>SNAMKLASKTAIVTGAARGIGFGIAQVLAREGARVIIADRDAHGEAAAASLRESGAQALFISCNIAEKTQVEALFSQAEEAFGPVDILVNNAGINRDAMLHKLTEADWDTVIDVNLKGTFLCMQQAAIRMRERGAGRIINIASASWLGNVGQTNYSASKAGVVGMTKTACRELAKKGVTVNAICPGFIDTDMTRGV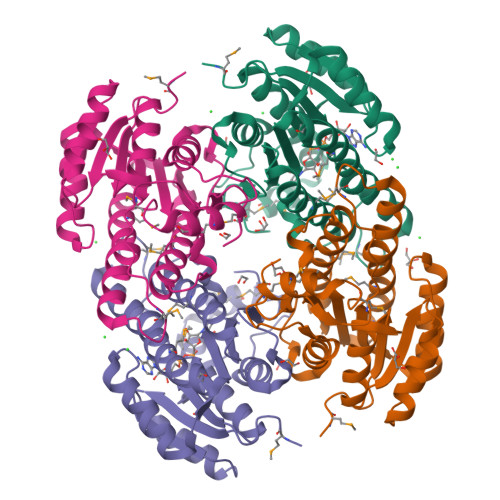PENVWQIMVSKIPAGYAGEAKDVGECVAFLASDGARYINGEVINVGGGMVL[8x]Phage satellite P4 polarity suppression protein, Psu, a building block of the viral capsid, inhibits hexameric transcription termination factor, ρ, by presently unknown mechanisms. The ρ hexamer adopts an NTPase-inactive, washer-like, open-ring conformation until NTPs (preferentially ATP) are engaged and RNA is bound at the SBS, leading to ring closure and RNA entrapment inside the ring. Our cryogenic electron microscopy structures of ρ-Psu complexes show that Psu dimers clamp two inactive, open ρ rings and promote their expansion to higher-oligomeric states. ATPase, nucleotide binding and nucleic acid binding studies revealed that Psu hinders ρ ring closure and traps nucleotides in their binding pockets on ρ.

In complex III, two hexameric ρ rings are bridged by six Psu dimers, that connect ρ(A) subunit 6 with ρ(B) subunit 1, ρ(A) subunit 5 with ρ(B) subunit 2, etc. Six Psu dimers bridge two open ρ hexamers, ρ(A) and ρ(B). ρ subunits are designated by increasing Arabic numerals from the centers to the peripheries of the complex. The different rotational orientations of the Psu-bridged ρ rings in complexes I, II, and III lead to different spacings between the innermost ρ subunits, which directly interact in complex I but are separated by a gap of ~ 30 Å and ~50 Å in complexes II and III, respectively. We further refined complex II (ATP; global resolution 3.8 Å), complex IIexpanded (ATP; global resolution 3.6 Å), complex III (ATPγS; global resolution 3.65 Å), and complex IIIexpanded (ATPγS; global resolution 4.25 Å). The ρ hexamers in complexes I, II and III exhibit slightly increased inter-subunit and ρ1-ρ6 rise values (8.4–8.8 Å and 42.2–43.9 Å, respectively). Psu interacts predominantly with one ρ CTD via the tip of its long coiled-coil (helices α1 and α2), the N-terminal part of helix α2 and the C-terminal helix α7. Psu helix α7 (residues 170–186) is placed in a cleft between the two neighboring ρ CTDs, covering the corresponding nucleotide-binding pocket. Psu R43 at the tip of the coiled-coil engages in cation-π interactions with Y197 of the main interacting ρ subunit. Finally, Psu P171, A172 and M175 (helix α7) engage in contacts with the T154-loop of the neighboring ρ subunit and cover the Watson-Crick side of the ATPγS base bound at that subunit, stabilizing it between ρ M186 and F355.

>[12x]MNLTELKNTPVSELITLGENMGLENLARMRKQDIIFAILKQHAKSGEDIFGDGVLEILQDGFGFLRSADSSYLAGPDDIYVSPSQIRRFNLRTGDTISGKIRPPKEGERYFALLKVNEVNFDKPENARNKILFENLTPLHANSRLRMERGNGSTEDLTARVLDLASPIGRGQRGLIVAPPKAGKTMLLQNIAQSIAYNHPDCVLMVLLIDERPEEVTEMQRLVKGEVVASTFDEPASRHVQVAEMVIEKAKRLVEHKKDVIILLDSITRLARAYNTVVPASGKVLTGGVDANALHRPKRFFGAARNVEEGGSLTIIATALIDTGSKMDEVIYEEFKGTGNMELHLSRKIAEKRVFPAIDYNRSGTRKEELLTTQEELQKMWILRKIIHPMGEIDAMEFLINKLAMTKTNDDFFEMMKRS;>[12x]MESTALQQAFDTCQNNKAAWLQRKNELAAAEQEYLRLLSGEGRNVSRLDELRNIIEVRKWQVNQAAGRYIRSHEAVQHISIRDRLNDFMQQHGTALAAALAPELMGYSELTAIARNCAIQRATDALREALLSWLAKGEKINYSAQDSDILTTIGFRPDVASVDDSREKFTPAQNMIFSRKSAQLASRQSV>MSTSSHTVLLIQTSPRLDSRTWGDYESVTDALDALCKMFEDFLSKKSAAPVTYDVSQVYEFLDKLSDVSMMIFNRETGQYIGRTRAWIKQQVYEMMRGRCQHPGSSGSSGSSGSSGSSGSSGSSEDIKDSVFKVLHAEEEPRGAD[2x]

By using functional proteomics, we and another group independently identified a piRNA biogenesis and chromosome segregation (PICS) complex (also named as PETISCO) that plays important roles in 21U-RNA biogenesis, chromosome segregation and cell division. The PICS complex is composed of TOFU-6, PICS-1 (also names as PID-3), ERH-2 and two mutually exclusive factors, PID-1 and TOST-1. The PID-1 containing complex is functional in piRNA maturation and processes piRNA precursors at 5′ termini via its association with IFE-3, while the TOST-1 containing form is essential for chromosome segregation and cell division in embryos. Complemented by biochemical and mutagenesis experiments, our structural biology data support that PICS is an octamer composed of two copies of each subunit, and unveil the assembly interface within PICS complex.

Then we fused a fragment of ERH-2 (1-103) with the EBM of PICS-1(PID-3) (180-200) via a (GSS)7 linker, crystallized the fusion protein, and solved its structure at a resolution of 2.40 Å. The overall structure is a tetramer formed by ERH-2 and EBM in a 2:2 ratio. In the structure, the ERH-2 homodimer adopts a butterfly-like architecture with the antiparallel β sheet from each protomer packed against each other. Two EBM molecules, named as EBMC and EBMD, respectively, are visible in the structure with each of them adopting a helix structure. The EBMC is accommodated into a v-shape concave via contacting with both ERH-2 molecules, ERH-2A and ERH-2B, respectively. EBMC mainly interacts with the β1, β2, α1, and α2 of ERH-2A, and extensive hydrophobic interactions are found throughout their binding interface. On one side, I182, V186, Phe187, and Leu190 of EBMC make hydrophobic interactions with Ile11, Thr13, Met38, Phe42, Phe61, and Leu65 of ERH-2A; on the other side, Val189 of EBMC is accommodated into a hydrophobic pocket composed of Ala34, Lys37, and Met38 of ERH-2A. Taken together, each EBM contacts with both protomers of ERH-2 dimer through both hydrophobic and hydrogen bonding interactions. ITC binding data indicate that neither of EBM double mutants, I182D/V186D and V189D/L190D, displayed ERH-2 binding affinity, which highlights  the roles of  hydrophobic residues in binding to ERH-2. We found that the three mutants disrupting the ERH-2/PICS-1 interaction, including I182D/V186D and V189D/L190D of PICS-1(PID-3), and M38D of ERH-2, all display abnormal chromosome segregation and cell division.>GFKQDIATIRGDLRTYAQDIFLAFLNKYPDERRYFKNYVGKSDQELKSMAKFGDHTEKVFNLMMEVADRATDCVPLASDANTLVQEKQHSSLTTGNFEKLFVALVEYMRASGQSFDSQSWDRFGKNLVSALSSAGMK[2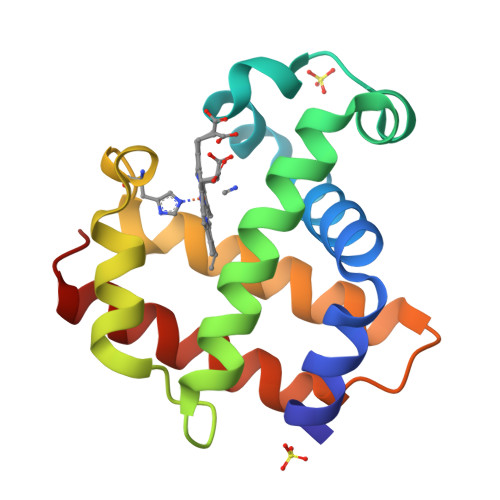x]> RSMAAGFKTVEPLEYYRRFLKENCRPDGRELGEFRTTTVNIGSISTADGSALVKLGNTTVICGVKAEFAAPSTDAPDKGYVVPNVDLPPLCSSRFRSGPPGEEAQV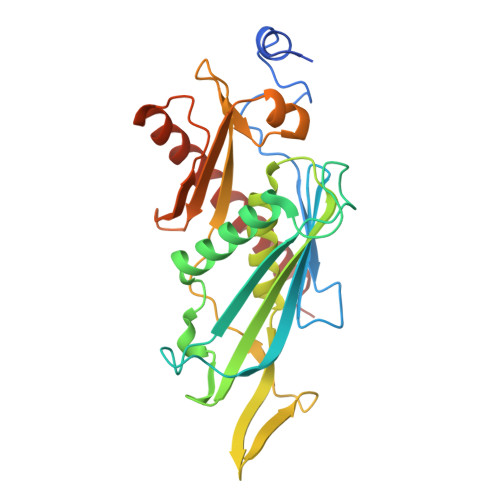ASQFIADVIENSQIIQKEDLCISPGKLVWVLYCDLICLDYDGNILDACTFALLAALKNVQLPEVTINEETALAEVNLKKKSYLNIRTHPVATSFAVFDDTLLIVDPTGEEEHLATGTLTIVMDEEGKLCCLHKPGGSGLTGAKLQDCMSRAVTRHKEVKKLMDEVIKSMKPK> MSETNTTDAKTVPAEAEKKKEQSLPFFKLFSFADKFDYLLMFVGSLGAIVHGSSMPVFFLLFGQMVNGFGKNQMDLHQMVHEVSRYSLYFVYLGLVVCFSSYAEIACWMYSGERQVAALRKKYLEAVLKQDVGFFDTDARTGDIVFSVSTDTLLVQDAISEKVGNFIHYLSTFLAGLVVGFVSAWKLALLSVAVIPGIAFAGGLYAYTLTGITSKSRESYANAGVIAEQAIAQVRTVYSYVGESKALNAYSDAIQYTLKLGYKAGMAKGLGLGCTYGIACMSWALVFWYAGVFIRNGQTDGGKAFTAIFSAIVGGMSLGQSFSNLGAFSKGKAAGYKLMEIINQRPTIIQDPLDGKCLDQVHGNIEFKDVTFSYPSRPDVMIFRNFNIFFPSGKTVAVVGGSGSGKSTVVSLIERFYDPNSGQILLDGVEIKTLQLKFLREQIGLVNQEPALFATTILENILYGKPDATMVEVEAAASAANAHSFITLLPKGYDTQVGERGVQLSGGQKQRIAIARAMLKDPKILLLDEATSALDASSESIVQEALDRVMVGRTTVVVAHRLCTIRNVDSIAVIQQGQVVETGTHEELIAKSGAYASLIR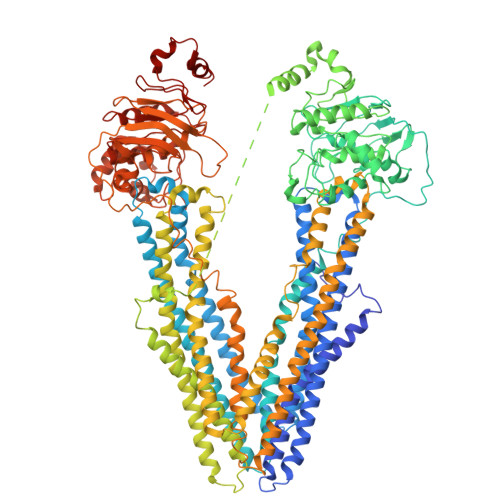FQEMVGTRDFSNPSTRRTRSTRLSHSLSTKSLSLRSGSLRNLSYSYSTGADGRIEMISNAETDRKTRAPENYFYRLLKLNSPEWPYSIMGAVGSILSGFIGPTFAIVMSNMIEVFYYTDYDSMERKTKEYVFIYIGAGLYAVGAYLIQHYFFSIMGENLTTRVRRMMLSAILRNEVGWFDEDEHNSSLIAARLATDAADVKSAIAERISVILQNMTSLLTSFIVAFIVEWRVSLLILGTFPLLVLANFAQQLSLKGFAGDTAKAHAKTSMIAGEGVSNIRTVAAFNAQSKILSLFCHELRVPQKRSLYRSQTSGFLFGLSQLALYGSEALILWYGAHLVSKGVSTFSKVIKVFVVLVITANSVAETVSLAPEIIRGGEAVGSVFSVLDRQTRIDPDDADADPVETIRGDIEFRHVDFAYPSRPDVMVFRDFNLRIRAGHSQALVGASGSGKSSVIAMIERFYDPLAGKVMIDGKDIRRLNLKSLRLKIGLVQQEPALFAATIFDNIAYGKDGATESEVIDAARAANAHGFISGLPEGYKTPVGERGVQLSGGQKQRIAIARAVLKNPTVLLLDEATSALDAESECVLQEALERLMRGRTTVVVAHRLSTIRGVDCIGVIQDGRIVEQGSHSELVSRPEGAYSRLLQLQTHRI> GSHMPVIAAPSM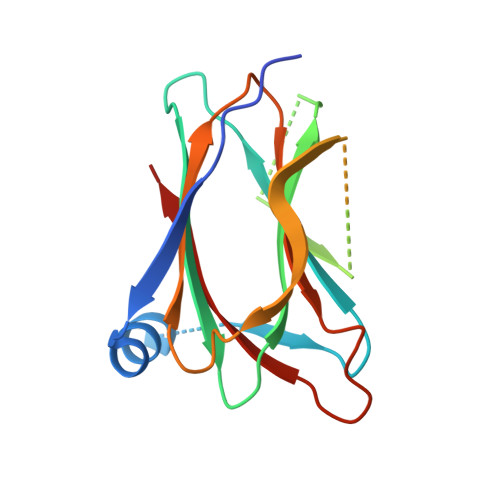WTRPQIKDFKEKIQQDADSVITVGRGEVVTVRVPTHEEGSYLFWEFATDNYDIGFGVYFEWTDSPNTAVSVHVSESSDDDEEEEENIGCEEKAKKNANKPLLDEIVPVYRRDCHEEVYAGSHQYPGRGVYLLKFDNSYSLWRSKSVYYRVYYTR>[6x]MASSHHHHHHHENLYFQGMTDTEVAQITDNPYKADFPILAANPKVAYLDSAATSQRPRVVIEAQSRFYETMNANALRGLYRWSVDATAAIEDARASIAKFIGAVDKNAKPESQQIIFTRNTSEALNLVASSLGRYALKPGDDVVISIMEHHSNIIPWQQICKATGANLVYLRMNSQYQITPEEIASKITERAKIV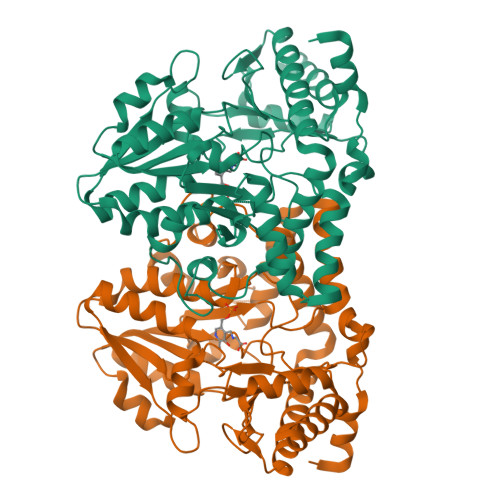SVTHVSNVLGTRNDIKAIAKRTHAMGAYMVVDAAQSAPHILVNVHDLDCDLLAFSAHRMCGPMGIGVLWGRAELLNAMPPFLTGGEMIDSVTETGAVWAPVPEKFEAGTQDAAGIYATGAAIKYLNGLDMAKIEKREELLARYLVQQLCTLDFVDIVGSKLGQNHVGAVAFNVRGVHPHDVSSILDMNNVCIRAGHHCAEPLLIELHESSTCRASVAFYNDKHDIDQLIEGLNQVWKIFGSAVNTKQNKELK>GPMTDISMGDLHANALLFLNILVRQGIIAISPENYAKFAEIYTLPELQADYWGTEAPVFSAENKQERLEEIKKQYNALIAQIKIINTKKLIRLIGDELVDRGVIDYFILKLLQALYDQGADFEILLSNHGIEFVEACELFKENGNKLVAKRLGNIQHGNSFHALQEAIAAGAISNEEVLNIYHQVYKKHLKIISYSLDPDANEIKVFSHAGIGLNHIRGLAR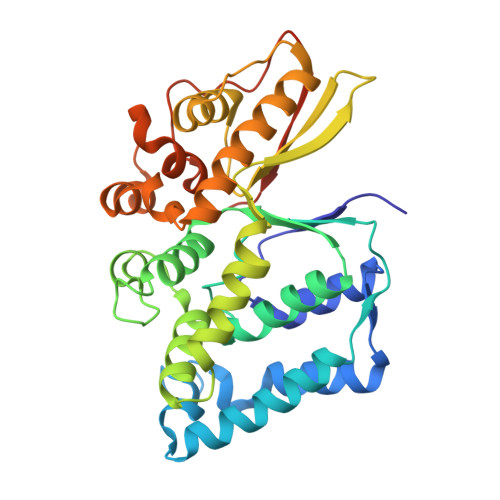KFKVPYSEESAVDLAKTIDAINKKFAEKASSGEIHTLYTHDMMYRGYAGEHLNSTDEVVAATVWGREYGDLIRTSKKFKITFIHGHDSYDPEKVEHVTLN[2x]[(1S)-1-chloroethyl]benzene | 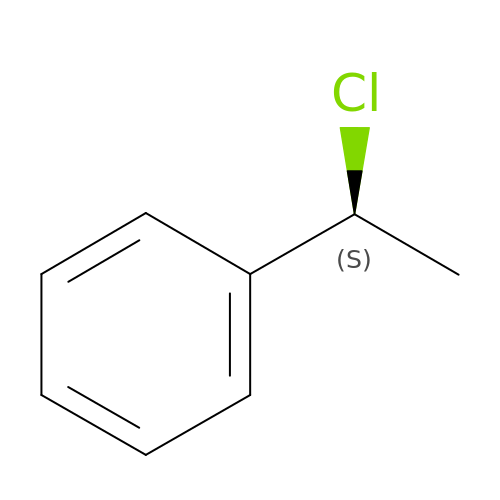C8 H9 Cl | GTLWADFFABIGAE-ZETCQYMHSA-N>[2x]MGKESTEQVASGLMCIGVTGHYDKTL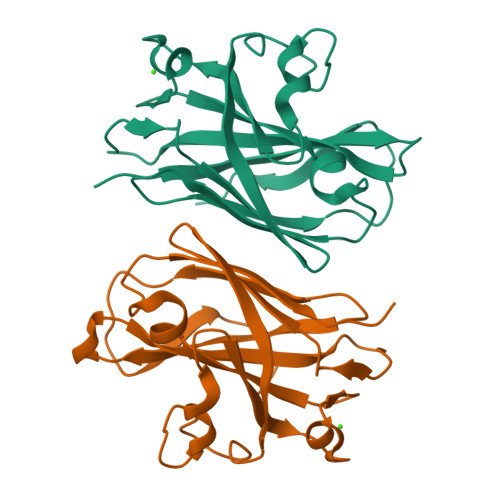GGIDKLAIYITPNAGSAPIDLKNAKLFLIYDGESHVLNYSTVTTATLGADDIFNSSAITDWSLADSSSYVVGVIQDADGSLSNGVINKGDIAVLLVNANAVFNKAIPTRSEVSGQFQPEFGAPAVIQFTTPAAYTQTVIELQHHHHHH> GSVYPKELTQVFEHYINNNLFDIDSLVKFIEELGYNLEDLATLCLAHLLGYKKLEEPLKREDFLSTWFMQGCSTISDMQECIKTLDVKLHEDLQYFTQIYNYAFNLILDPNRKDIDTDEGIQYWKLFFQPEYPVRMEPDLLEAWFRFLRDEGKTTISKDTWRMLLLFFKRYPTIQKIISDYDETAAWPFIIDEFYECLQDQQ;> GSNKRLTEDERIEKELNTER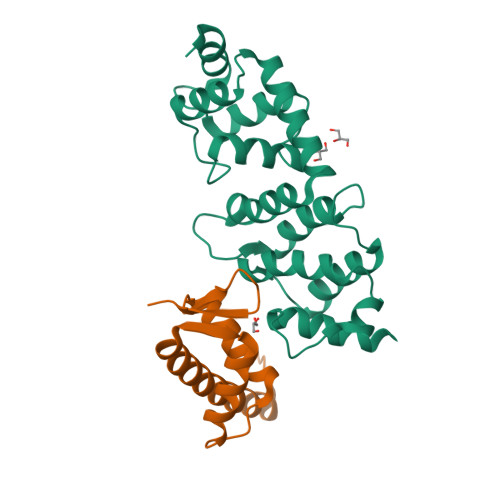QIFLEACIVRIMKAKRNLPHTTLVNECIAQSHQRFNAKVSMVKRAIDSLIQKGYLQRGDDGESYAYLA>MPMVLLECDKDIPERQKHIYLKAPNEDTREFLPIAN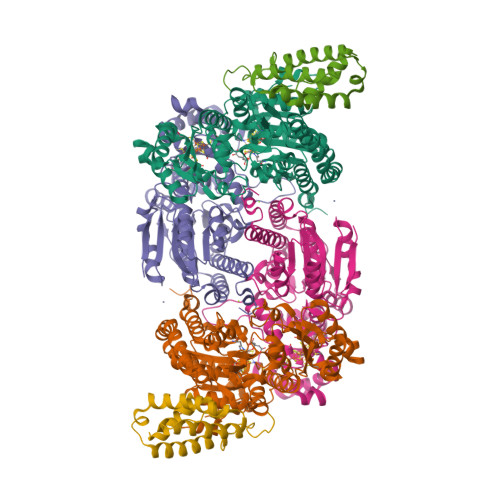AATIPGTLSERGCAFCGAKLVIGGVLKDTIQMIHGPLGCAYDTWHTKRYPTDNGHFNMKYVWSTDMKESHVVFGGEKRLEKSMHEAFDEMPDIKRMIVYTTCPTALIGDDIKAVAKKVMKDRPDVDVFTVECPGFSGVSQSKGHHVLNIGWINEKVETMEKEITSEYTMNFIGDFNIQGDTQLLQTYWDRLGIQVVAHFTGNGTYDDLRCMHQAQLNVVNCARSSGYIANELKKRYGIPRLDIDSWGFNYMAEGIRKICAFFGIEEKGEELIAEEYAKWKPKLDWYKERLQGKKMAIWTGGPRLWHWTKSVEDDLGVQVVAMSSKFGHEEDFEKVIARGKEGTYYIDDGNELEFFEIIDLVKPDVIFTGPRVGELVKKLHIPYVNGHGYHNGPYMGFEGFVNLARDMYNAVHNPLRHLAAVDIRDKSQTTPVIVRGAA[2x];>MSNCELTVLKPAEVKLSPRDREGIINPMYDCQPAGAQYAGIGIKDCIPLVHGGQGCTMFVRLLFAQHFKENFDVASTSLHEESAVFGGAKRVEEGVLVLARRYPNLRVIPIITTCSTEVIGDDIEGSIRVCNRALEAEFPDRKIYLAPVHTPSFKGSHVTGYAECVKSVFKTITDAHGKGQPSGKLNVFPGWVNPGDVVLLKRYFKEMDVEANIYMDTEDFDSPMLPNKSIETHGRTTVEDIADSANALATLSLARYEGNTTGELLQKTFAVPNALVNTPYGIKNTDDMLRKIAEVTGKEIPESLVRERGIALDALADLAHMFFANKKVAIFGHPDLVLGLAQFCMEVELEPVLLLIGDDQGNKYKKDPRIEELKNTAHFDIEIVHNADLWELEKRINAGLQLDLIMGHSKGRYVAIEANIPMVRVGFPTFDRAGLYRKPSIGYQGAMELGEMIANAMFAHMEYTRNKEWILNTW[2x];>[2x]MSQSHLDDLFAYVEERCLWQFFSRTWDREENIEGVLNQVGRLLTGQEPLRGTPQERLFYADALAMANDVRERFPWASQVNKEEIEFLLDGLKSRLVDVTITRSTNRELNHHLY>GPNLELLESFGQNYPEEADGTLDCISMALTCTFNRWGTLLAVGCNDGRIVIWDFLTRGIAKIISAHIHPVCSLCWSRDGHKLVSASTDNIVSQWDVLSGDCDQRFRFPSPILKVQYHPRDQNKVLVCPMKSAPVMLTLSDSKHVVLPVDDDSDLNVVASFDRRGEYIYTGNAKGKILVLKTDSQDLVASFRVTTGTSNTTAIKSIEFARKGSCFLINTADRIIRVYDGREILTCGRDGEPEPMQKLQDLVNRTPWKKCCFSGDGEYIVAGSARQHALYIWEKSIGNLVKILHGTRGELLLDVAWHPVRPIIASISSGVVSIWAQNQVENWSAFAPDFKELDENVEYEERESEFDIEDEDKSEPKQTGADAAEDEEVDVTSV[2x];> EPKQTG

The multi-protein complex WRAD, formed by WDR5, RbBP5, Ash2L and Dpy30, binds to the MLL SET domain to stabilize the catalytically active conformation required for histone H3K4 methylation. RbBP5 is central to MLL catalytic activation, by making critical contacts with the other members of the complex. The amino terminus of RbBP5, residues 1–325, is composed of a series of canonical WD40 repeats that are predicted to form a seven bladed β-propeller domain, which is the major structural feature of the protein. However, it is the region immediately following this domain, residues 340–380, that stimulates methyltransferase activity through cooperative interactions with the other members of WRAD complex and the MLL SET domain.

After screening a wide range of constructs, diffracting crystals of the RbBP51–380 construct were obtained, which contains both the β-propeller and the regions known to interact with other members of the MLL complex. The structure was determined by molecular replacement, for details see ‘Materials and Methods’ section, and refined to a resolution of 2.5Å. The asymmetric unit contains two copies of the construct, and data collection and refinement statistics are presented in Table 1. The β-propeller domain structure is basically consistent between both copies, but the 325–380 region is largely disordered and varies significantly. The two copies of the β-propeller are linked in the crystal structure due to a strand swap which disrupts the seventh blade of the copy B propeller. RbBP5 forms a canonical seven bladed WD40 repeat β-propeller in which the seventh blade is formed from three anti-parallel strands from the C-terminal region of the domain and is completed with a strand originating from the N-terminus of the domain. Between the third and fourth strands of the 5th propeller blade there is an insert which includes a short α-helix, which lies on one face of the propeller toward the rim. A conspicuous feature of the RbBP5 β-propeller, which appears to be quite distinct from other WD40 proteins in chromatin modification complexes such as WDR5 in MLL and EED and RbAp48 in PRC2, is that the central axis is not formed from bulky aromatic side chains, but instead polar residues dominate the propeller axis. On the ‘top’ face, defined as the face containing the α-helical insert, the propeller axis has a complete ring of basic side-chains, which extends into a basic groove between blades six and seven, and so reaches toward the edge of the propeller.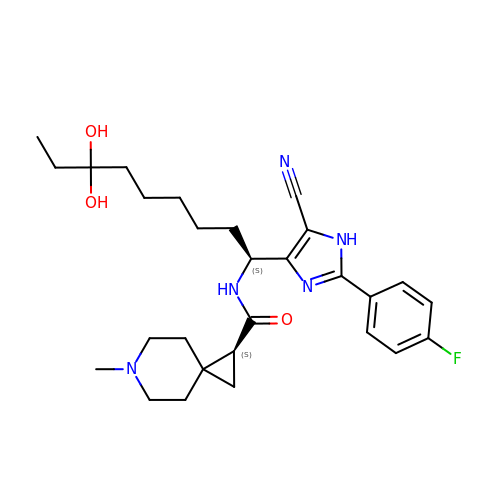(1S)-N-{(1S)-1-[5-cyano-2-(4-fluorophenyl)-1H-imidazol-4-yl]-7,7-dihydroxynonyl}-6-methyl-6-azaspiro[2.5]octane-1-carboxamide | C28 H38 F N5 O3 | HQQQLMWKYHVCDC-YADHBBJMSA-N> MAKLGIH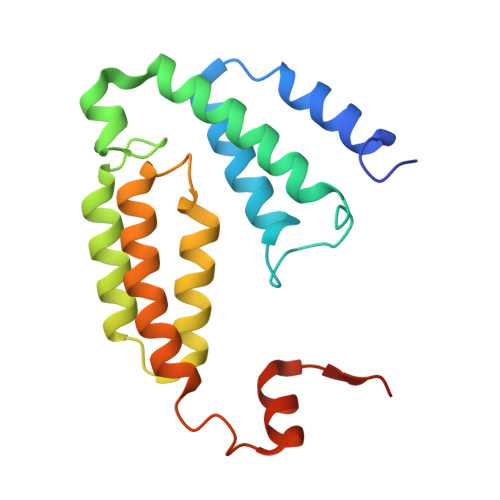SNDTRDAWVNKIAQLNTLEKAAEMLKQFRMDHTTPFRNSYELDNDYLWIEAKLEEKVAVLKARAFNEVDFRHKTAFGEDAKSVLDGTVAKMNAAKDKWEAEKIHIGFRQAYKPPIMPVNYFLDGERQLGTRLMELRNLNYYDTPLEELRKQRGVRVVHLQSPH> GPMDGTAAEPRPGAGSLQHAQPPPQPRKKRPEDFKFGKILGEGSFSTVVLARELATSREYAIKILEKRHIIKENKVPYVTRERDVMSRLDHPFFVKLYFTFQDDEKLYFGLSYAKNGELLKYIRKIGSFDETCTRFYTAEIVSALEYLHGKGIIHRDLKPENILLNEDMHIQITDFGTAKVLSPESKQARANSFVGTAQYVSPELLTEKSACKSSDLWALGCIIYQLVAGLPPFRAGNEYLIFQKIIKLEYDF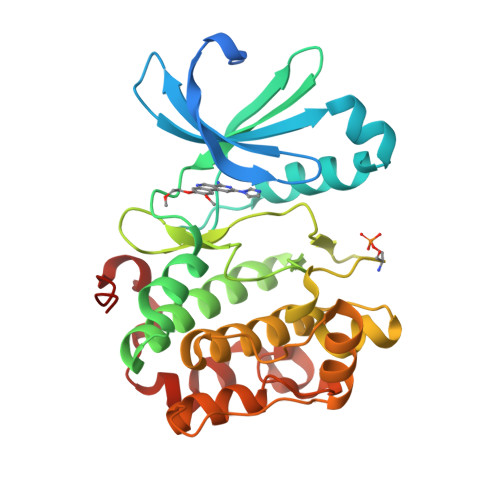PEKFFPKARDLVEKLLVLDATKRLGCEEMEGYGPLKAHPFFESVTWENLHQQTPPKLT> ADLPAPDDTGLQAVLHTALSQGAPGAMVRVDDNGTIHQLSEGVADRATGRAITTTDRFRVGSVTKSFSAVVLLQLV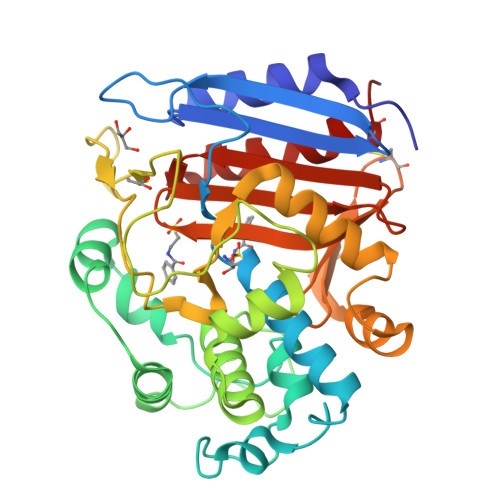DEGKLDLDASVNTYLPGLLPDDRITVRQVMSHRSGLYDYTNDMFAQTVPGFESVRNKVFSYQDLITLSLKHGVTNAPGAAYSYSNTNFVVAGMLIEKLTGHSVATEYQNRIFTPLNLTDTFYVHPDTVIPGTHANGYLTPDEAGGALVDSTEQTVSWAQSAGAVISSTQDLDTFFSALMSGQLMSAAQLAQMQQWTTVNSTQGYGLGLRRRDLSCGISVYGHTGTVQGYYTYAFASKDGKRSVTALANTSNNVNVLNTMARTLESAFCGKPTT> GGACAUAUAAACGCGUGGAUAUGGCACGCGAGUUUCUACCGGGCACCGUAAAUGUC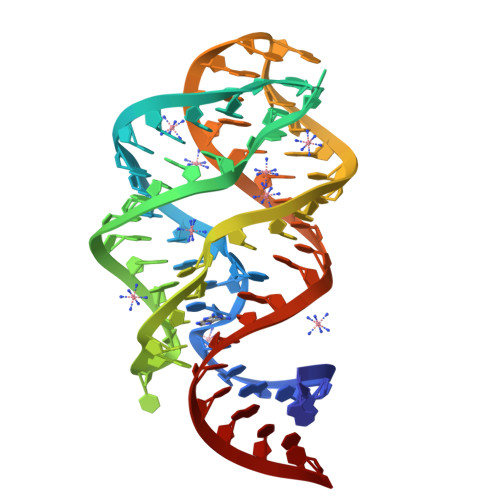CGAUUAUGUCC In this article, we studied five members of the PLL lectin family from P. laumondii subsp. laumondii TT01 (PLL, PLL2, PLL3, PLL4, PLL5, collectively referred to as PLLs). All studied lectins belong to the seven-bladed β-propeller structural family. Each blade makes a W-motif composed of four antiparallel beta-strands (β1-β4) connected by β-turns and loops. The saccharide binding sites are located between the adjacent blades and are uniquely organized in two separate circles around the monomer.

The newly characterized lectins PLL, PLL4, and PLL5 were produced recombinantly in Escherichia coli and were purified by affinity chromatography. The PLL chain A blade W1 interacts with chain B blade W3, whereas in the case of PLL2, PLL4 and PLL5, chain A blade W1 interacts with chain B blade W5. The PLL is a tetramer in solution (sedimentation coefficient 7.6 S); PLL4 and PLL5 form dimers in solution (sedimentation coefficients: PLL4 = 4.9 S and PLL5 = 4.7 S). PLL preferred branched fucosylated saccharides (BLeY and ALeY); PLL4 and PLL5 preferred MGMR. The PLL5 gene exhibited negligible expression under the conditions tested, raising questions about its inducibility. Among the PLL family, PLL5 had the most pronounced effect on basal PO activity (one-way ANOVA, P-value <0.001), elevating it to levels comparable to those seen with full activation of the PO system. Nonetheless, the extent of PLL5-induced melanisation under natural infection is uncertain due to low pll5 gene expression in early bacterial growth stages. Interestingly, PLL5 was observed to reduce ROS production in PMA-induced response, although a significant variability was noted among blood samples, likely reflecting inter-individual differences among blood donors. The mechanism by which PLL5 inhibits PMA-induced ROS production remains unknown, but it highlights PLL5’s unique activity among other PLLs.

>MKKEPIKTSNPDNTESSDANEVEIENPTIAASGIVSVANTSDGRIEVFGVGGDNAVWRNGQTTHTGASWTGWSSLGGSVTSKPAAYLNSDGRLEVFVRGSDNALWHNWQTTPNASWSGWQSLGGALTSNPAVYINADGRLEVFARGLDNTLWHIWQTAPHSNPWSSWYSLGHVITSNPAVHINADGRLEVFARGADNALWHIWQTAPHSGYWSGWHSLGGVLSSDPVVARTVDGRLEVFVRAVDNALWHIWQTAPNSSQWSNWASLGGTITSAPAVIKYFDNRLVVFARAIDNALWHIWQNDTHSGSWSNWGSLGGGLSSGPDVVENANGYIEVFVRATDNALWNIKRTSPSSWSSWASLGGTLIDASAIK[4x]> MKSSGA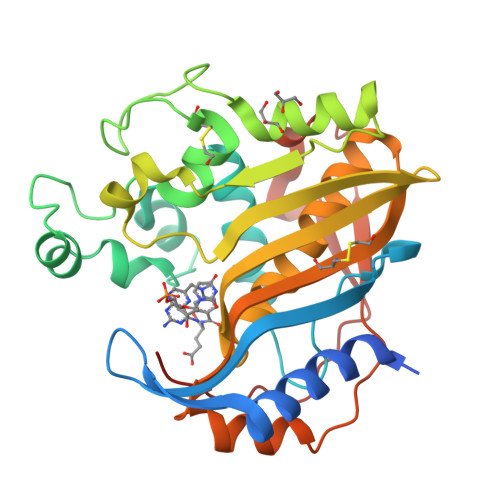HGNVMGDAGVLKNEDESKYLDQVRYILKNGERIDDRTGAGTISVFGMHSVYSLRNGVVPVLTTKRVYWKGVVEELLWFIRGDTNAKHLSEKGVRIWDANGSRQFLDQCGFSDRSEGDLGPIYGFQWRHCGAEYRGMDTDYTNQGIDQLSEIIDLIKNEPHSRRIILSAWNVKDLKLMALPPCHTLAQFAVRNGELSCQLYQRSGDMGLGVPFNLASYGLLTHMIAHVCGLKTGHLCHVLGDAHVYMNHVDALQEQLKRQPRQFPTVRFIGNIKTIDDFTYESIVLENYQPMPAIKMAMAV>SNAMVLGKPQTDPTLEWFLSHCHIHKYPSKSTLIHQGEKAETLYYIVKGSVAVLIKDEEGKEMILSYLNQGDFIGELGLFEEGQERSAWVRAKTACEVAEISYKKFRQLIQVNPDILMRLSSQMANRLQITSEKVGNLAFLDVTGRIAQTLLNLAKQP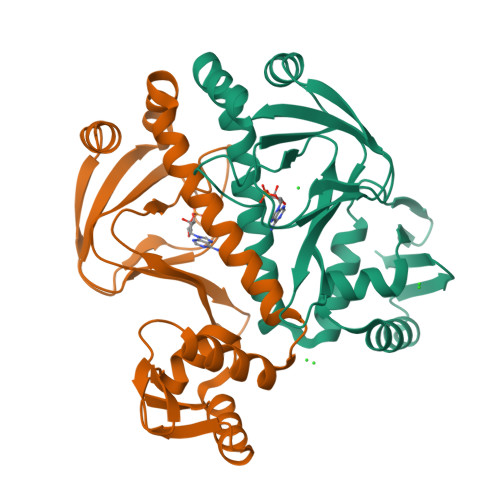DAMTHPDGMQIKITRQEIGQIVGCSRETVGRILKMLEDQNLISAHGKTIVVYGTR[2x]> MQIPL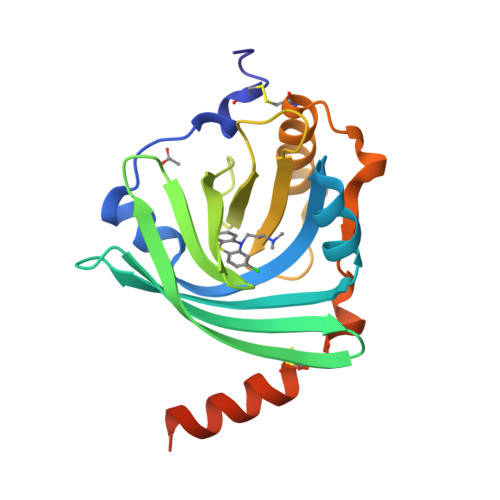CANLVPVPITNATLDRITGKWFYIASAFRNEEYNKSVQEIQATFFYFTPNKTEDTIFLREYQTRQNQCFYNSSYLNVQRENGTVSRYEGGREHVAHLLFLRDTKTLMFGSYLDDEKNWGLSFYADKPETTKEQLGEFYEALDCLRIPRSDVMYTDWKKDKCEPLEKQHEKERKQEEGESHHHHHH> MIVEKLVHVASVEKGRSYEDFQKVYNAIALKLREDDEYDNYIGYGPVLVRLAWHISGTWDKHDNTGGSYGGTYRFKKEFNDPSNAGLQNGFKFLEPIHKEFPWISSGDLFSLGG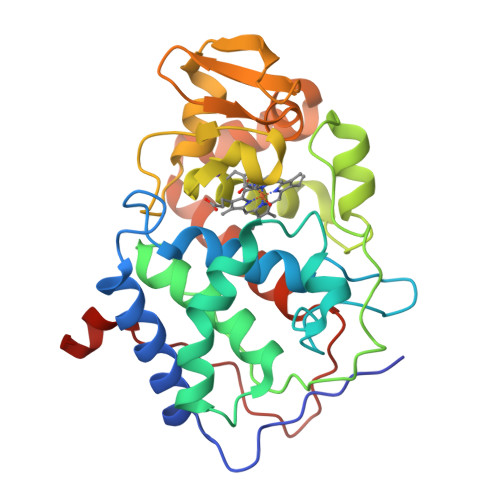VTAVQEMQGPKIPWRCGRVDTPEDTTPDNGRLPDADKDAGYVRTFFQRLNMNDREVVALMGAHALGKTHLKNSGYEGPQGAANNVFTNEFYLNLLNEDWKLEKNDANNEQWDSKSGYMMLPTDYSLIQDPKYLSIVKEYANDQDKFFKDFSKAFEKLLENGITFPKDAPSPFIFKTLEEQGL>[60x]MPAIRKARGWVPPGYNYLGPFNQDFNKKPTNPSDNAARKHDLEYNKLIKQGHNPYWNYNHADEDFIKETDQATDWGGKFGNFVFRAKRALAPELAPPAKKKTKTKHTEPEYSHKHIKAGTKRGKPFYLFVNLARKKARMTDTQDVSEQQSDQPSVASTNAKAGGGGGGGGSGVGHSTGNYNNRTEFYYHGDEVTIVCHSSRHIHLNMSESEEYKIYDTDRGPRFPTDQTLQGRDTINDS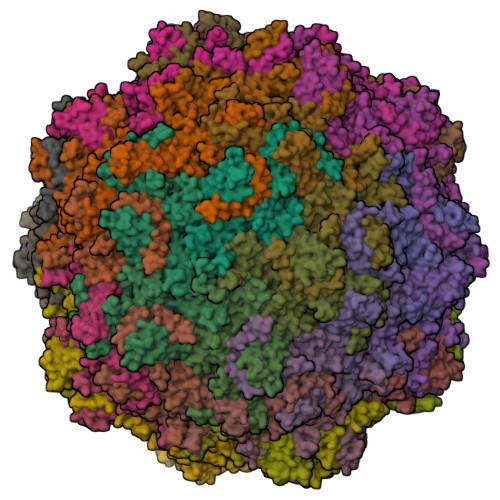YHAQVETPWFLINPNSWGTWMNPADFQQLTTTCREVTLEHLDQTLDNIVIKTVSKQGSGAEETTQYNNDLTALLQVALDKSNQLPWVADNMYLDSLGYIPWRPCKLKQYSYHVNFWNTIDIISGPQQNQWQQVKKEIRWDDLQFTPIETTTEIDLLRTGDSWTSGPYKFNTKPTQLSYHWQSTRHTGSVHPTDPPNAIGQQGQNIRDINGWQWGDRSDPMSAATRVSNFHIGYSWPEWRIHYGSGGPAINPGAPFSQAPWSTDPQVRLTQGASEKAIFDYNHGDDDPAHRDQWWQNNLPITGQTNWAPKNAHQANLSSNVPSRQEFWTQDYHNTFGPFTAVDDVGIQYPWGAIWTKTPDTTHKPMMSAHAPFICKDGPPGQLLVKLAPNYTENLQTDGLGNNRIVTYATFWWTGKLILKGKLRLPRQFNLYNLPGRPRGTEAKKFLPNEIGHFELPFMPGRCMPNYTM> METVYCTFDHKLSLSDISTLCKLMNIVIPIPAHHHLIGSGNLGLYPIVSSNKDYVHIRNVLRTMVVTILQKVEGNQLVLRKPMTGQQYAIKNTGPFPWEKGDTLTLIPPLSTHSEEKLLKLGDWELTVPLVVPTAIAAEINIRLLCIGLIAVHREYNEMQTIIDELCSIQYRDVLIKLPDIVNDKQSMYSMKTACISLSMITAMAPDIVRTYIDRLTLEDHSMLLIKCQELLSKRTTLSTQRCGQLHATDIKDELKKIKSVLTMIDQINSLTNEKTYFVVCDVSADNRMATCIYK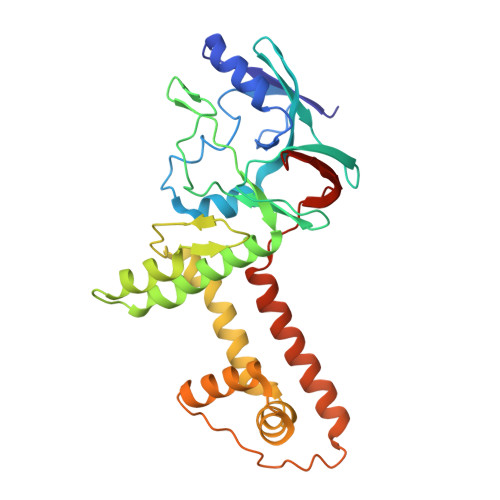N>[2x]MIKPVGSDELRPRFVYDPEQHHRLSSEAESLPSVIVSSQAAGNAVMLGAGYFSPLDGFMNLADALSSAQSMTLTDGRFFPVPLLCLLESADAIAGATRIALRDPNVEGNPVLAVMDVTAVEQVSDAQMALMTEQVYGTSDPKHPGVETFNSQGRTAISGPIQVLNFSYFQTDFPDTFRTAVEIRHEIQERGWQKIVAFQTRNPMHRAHEELCKMAMEAVEADGVVIHMLLGQLKPGDIPAPV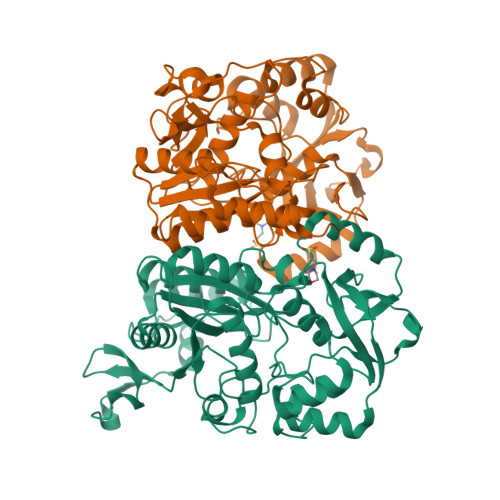RDAAIRTMAELYFPPNTVMVTGYGFDMLYAGPREAVLHAYFRQNMGATHFIIGRDHAGVGDYYGPFDAQTIFDDAVPTDVLAIEIFRADNTAYSKKLGRVVMMRDAPDHTPDDFIQLSGTRVREMLGQGEAPPPEFSRPEVAQILMDYYRSLPQS[5-methoxy-2-({[4-(trifluoromethyl)benzyl]sulfonyl}carbamoyl)-1H-indol-1-yl]acetic acid | C20 H17 F3 N2 O6 S | 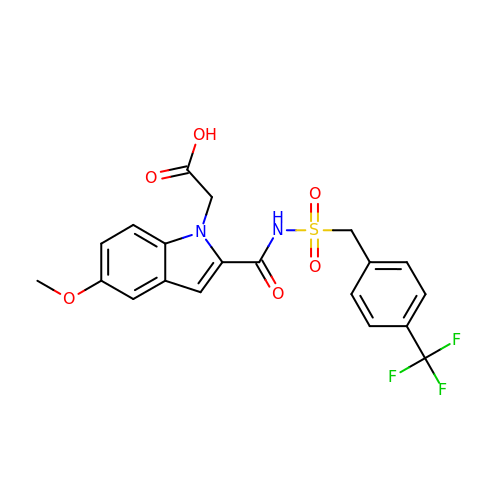BCONJIVPNWPJDO-UHFFFAOYSA-N>MSYYHHHHHHLESTSLYKKAGLDYDIPTTENLYFQGMNTLREV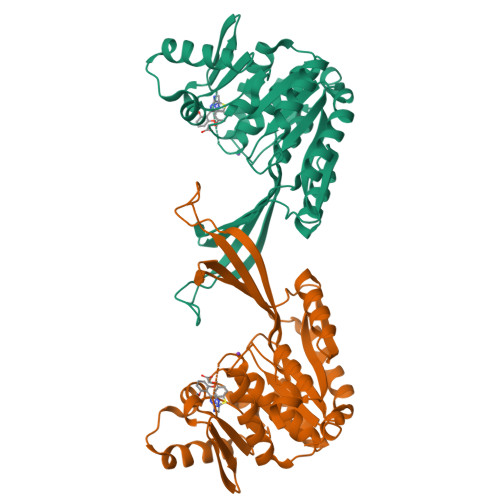VPVPREQLARSRVLVVGDVMLDRYWFGNVDRISPEAPVPVVHVQRQEERLGGAANVARNAVTLGGQAGLLCVVGCDEPGERIVELLGSSGVTPHLERDPALPTTIKLRVLARQQQLLRVDFEAMPTHEVLLAGLARFDVLLPQHDVVLMSDYAKGGLTHVTTMIEKARAAGKAVLVDPKGDDWARYRGASLITPNRAELREVVGQWKSEDDLRARVANLRAELDIDALLLTRSEEGMTLFSAGGELHAPALAREVFDVSGAGDTVIATVATMLGAGVPLVDAVVLANRAAGIVVGKLGTATVDYDELFH[2x]> GDPIADMIDQTVNNQ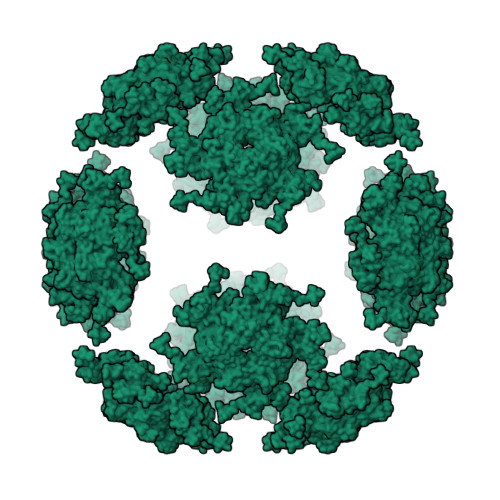VNRSLTALQVLPTAANTEASSHRLGTGVVPALQAAETGASSNASDKNLIETRCVLNHHSTQETAIGNFFSRAGLVSIITMPTTGTQNTDGYVNWDIDLMGYAQLRRKCELFTYMRFDAEFTFVVAKPNGELVPQLLQYMYVPPGAPKPTSRDSFAWQTATNPSVFVKMTDPPAQVSVPFMSPASAYQWFYDGYPTFGEHLQANDLDYGQCPNNMMGTFSIRTVGIEKSPHSITLRVYMRIKHVRAWIPRPLRNQPYLFKTNPNYKGNDIKCTSTSRDKITTL4'-ethylthymidine 5'-(tetrahydrogen triphosphate) | C12 H21 N2 O14 P3 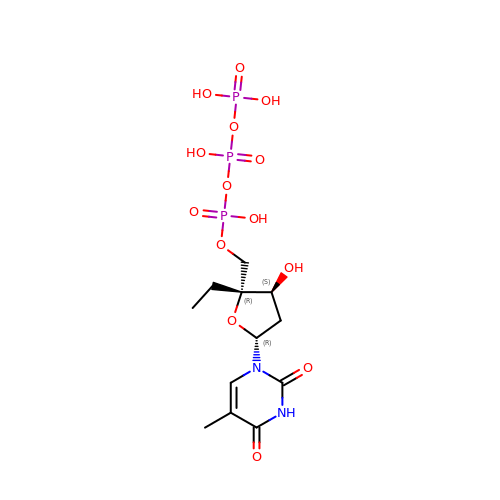| RICQFQMPHJAPNN-YGOYTEALSA-N> MSEFSQTALFPSLPRTARGTAVVLGNTPAGDKIQYCNGTSVYTVPVGSLTDTEIYTEHSHQTTVAKTSPSGYYCASGDVHGNVRIWDTTQTTHILKTTIPVFSGPVK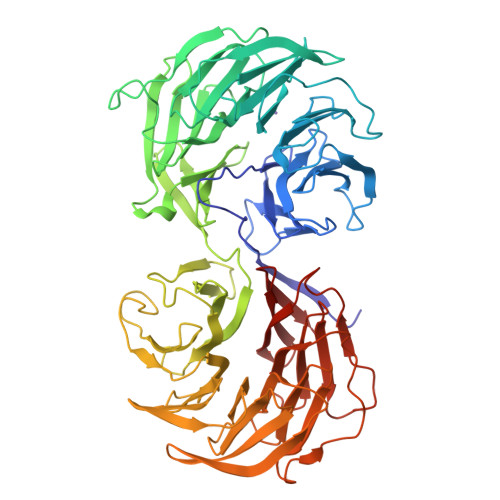DISWDSESKRIAAVGEGRERFGHVFLFDTGTSNGNLTGQARAMNSVDFKPSRPFRIISGSDDNTVAIFEGPPFKFKSTFGEHTKFVHSVRYNPDGSLFASTGGDGTIVLYNGVDGTKTGVFEDDSLKNVAHSGSVFGLTWSPDGTKIASASADKTIKIWNVATLKVEKTIPVGTRIEDQQLGIIWTKQALVSISANGFINFVNPELGSIDQVRYGHNKAITALSSSADGKTLFSADAEGHINSWDISTGISNRVFPDVHATMITGIKTTSKGDLFTVSWDDHLKVVPAGGSGVDSSKAVANKLSSQPLGLAVSADGDIAVAACYKHIAIYSHGKLTEVPISYNSSCVALSNDKQFVAVGGQDSKVHVYKLSGASVSEVKTIVHPAEITSVAFSNNGAFLVATDQSRKVIPYSVANNFELAHTNSWTFHTAKVACVSWSPDNVRLATGSLDNSVIVWNMNKPSDHPIIIKGAHAMSSVNSVIWLNETTIVSAGQDSNIKFWNVPF> MQAGKPILYSYFRSSCSWRVRIALALKGIDYKTVPINLIKDGGQQFSKDFQALNPMKQVPTLKIDGITIHQSLAIIEYLEETRPTPRLLPQDPKKRASVRMISDLIAGGIQPLQNLSVLKQVGEEMQLTWAQNAITCGFNALEQILQSTAGIYCVGDEVTMADLCLVPQVANAERFKVDLTPYPTISSINKRLLVLEAFQVSHPCR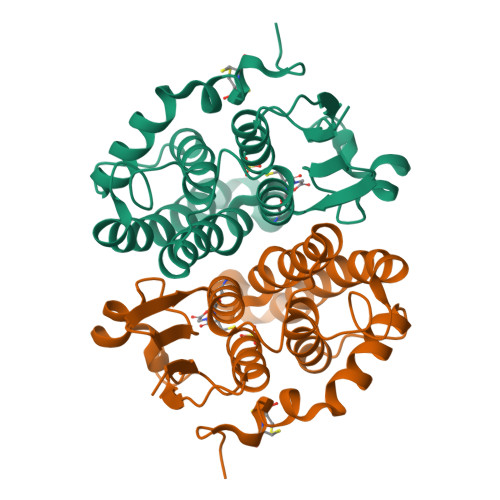QPDTPTELRA> MGYKEISLKYGKGAVDVKIDENMCTVLYPEDLPGVEDPMAEVSRSLKDPIGKAPLSDLVKGKKDVVILASDITRPSPSHILIPPITDELNRAGISDDSIKIVFGLGYHRKHTDDEKKTL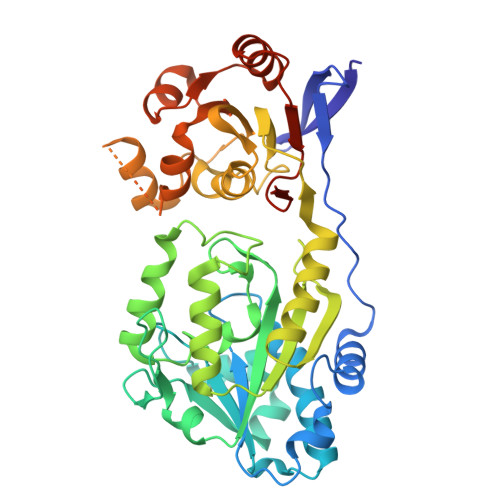VGEEVFNRIKCIDHDIDDCVYVGTTKRGTPVEVFREVYNADFIIATGNLELHYKAGYSGGHKALLPGVCSKNTIEKNHALMFSEGAMPGKIDGNPMREDIEEGGKLARVDFIVNAVLNSHKEIVKVVSGDPIKAHREGAKYIDKMYKRVIPEKADIVVASCGGYPKDINLYQAQKGLDNAQYSVKDGGTIILVAECREGLGEKLFSDWMVNSSSVDEPLKWIKEEFRLGAHKAAVICEVLKRADIYLISSFDRSLTEKIFFKYAKTPQDALDEAIKKYHDPKILVLPYANSTLPYVEEASWSHPQFEK> GSHMKNPYSNQIEREELILKYLPLVKAIATNIKKHLPEDVDIRDLISYGVIGLIKAVDNLSTENPKRAEAYIKLRIKGAIYDYLRSLDFGSRQVREKERRIKEVVEKLKEKLGREPTDEEVAKELGISTEELFKTLDKINFSYILSLEEVFRDFARDYSELIPSSTNVEEEV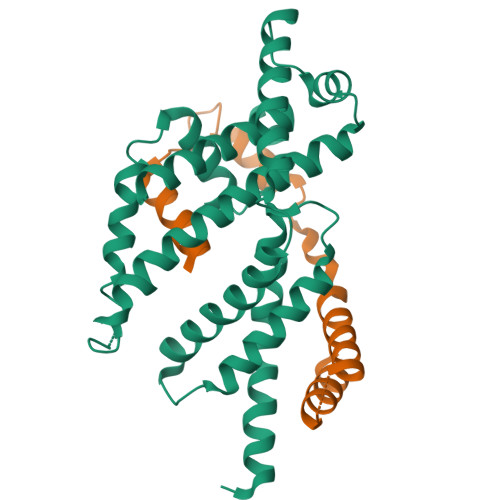IKRELTEKVKEAVSKLPEREKLVIQLIFYEELPAKEVAKILETSVSRVSQLKAKALERLREMLSNPL;> MVNRIELSRLIGLLLETEKRKNTEQKESGTNKIEDKVTLSKIAQELSKNDVEEKDLEKKVKELKEKIEKGEYEVSDEKVVKGLIEFFT> GSHMAIVKVTDADFDSKVESGVQLVDFWATWCGTCKMIAPVLEELAADYEGKADILKLDVDENPSTAAKYEVMSIPTLIVFKDGQPVDKVVGFQPKE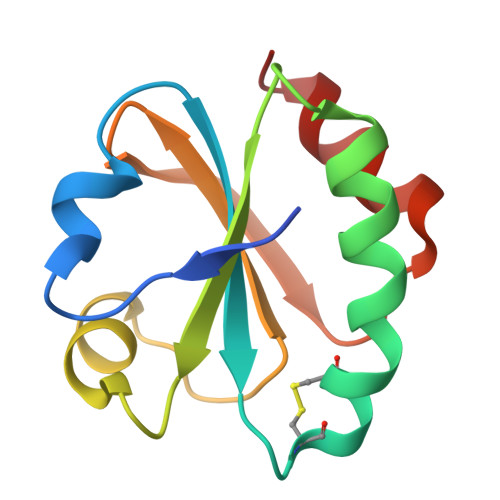NLAEVLDKHL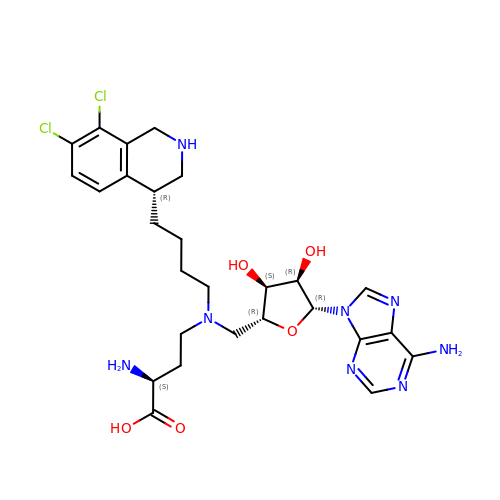5'-([(3S)-3-amino-3-carboxypropyl]{4-[(4R)-7,8-dichloro-1,2,3,4-tetrahydroisoquinolin-4-yl]butyl}amino)-5'-deoxyadenosine | C27 H36 Cl2 N8 O5 | VHXBLPZYVDYOPX-STPVDRQBSA-N> PCPGACVCYNEPKVTTSCPQQGLQAVPVGIP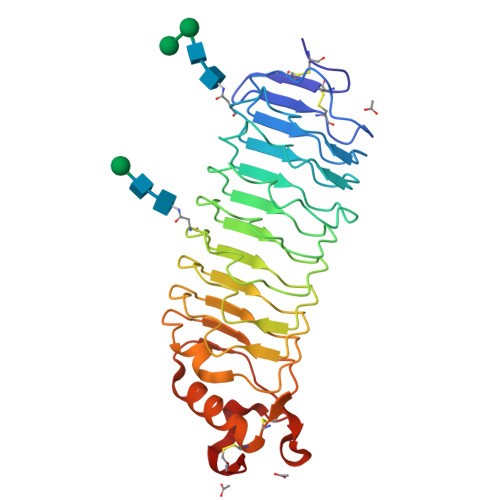AASQRIFLHGNRISHVPAASFRACRNLTILWLHSNVLARIDAAAFTGLALLEQLDLSDNAQLRSVDPATFHGLGRLHTLHLDRCGLQELGPGLFRGLAALQYLYLQDNALQALPDDTFRDLGNLTHLFLHGNRISSVPERAFRGLHSLDRLLLHQNRVAHVHPHAFRDLGRLMTLYLFANNLSALPTEALAPLRALQYLRLNDNPWVCDCRARPLWAWLQKFRGSSSEVPCSLPQRLAGRDLKRLAANDLQGCA> MRSPVR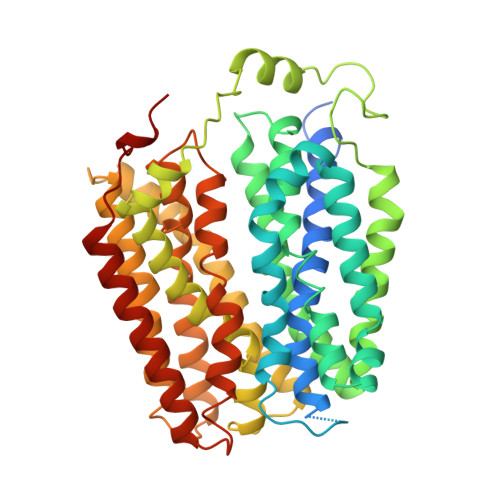DLARNDGEESTDRTPLLPGAPRAEAAPVCCSARYNLAILAFFGFFIVYALRVNLSVALVDMVDSNTTLEDNRTSKACPEHSAPIKVHHNQTGKKYQWDAETQGWILGSFFYGYIITQIPGGYVASKIGGKMLLGFGILGTAVLTLFTPIAADLGVGPLIVLRALEGLGEGVTFPAMHAMWSSWAPPLERSKLLSISYAGAQLGTVISLPLSGIICYYMNWTYVFYFFGTIGIFWFLLWIWLVSDTPQKHKRISHYEKEYILSSLRNQLSSQKSVPWVPILKSLPLWAIVVAHFSYNWTFYTLLTLLPTYMKEILRFNVQENGFLSSLPYLGSWLCMILSGQAADNLRAKWNFSTLCVRRIFSLIGMIGPAVFLVAAGFIGCDYSLAVAFLTISTTLGGFCSSGFSINHLDIAPSYAGILLGITNTFATIPGMVGPVIAKSLTPDNTVGEWQTVFYIAAAINVFGAIFFTLFAKGEVQNWALNDHHGHRH>MAYRKRGARRETNLKQDERMQEKEDSKNINNDSPKSQLSEKVLSKKEEIITDNQEEVKISDEVKKSNKEESKQLLEVLKTKEEHQKEVQYEILQKTIPTFEPKESILKKLEDIKPEQAKKQTKLFRIFEPKQLPIYRANGERELRNRWYWKLKRDTLPDGDYDVREYFLNLYDQVLMEMPDYLLLKDMAVENKNSRDAGKVVDSETAAICDAIFQDEETEGAVRRFIAEMRQRVQADRNVVNYPSILHPIDHAFNEYFLQHQLVEPLNNDIIFNYIPERIRNDVNYILNMDRNLPSTARYIRPNLLQDRLNLHDNFESLWDTITTSNYILARSVVPDLKELVSTEAQIQKMSQDLQLEALTIQSETQFLTGINSQAANDCFKTLIAAMLSQRTMSLDFVTTNYMSLISGMWLLTVIPNDMFIRESLVACQLAIINTIVYPAFGMQRMHYRNGDPQTPFQIAEQQIQNFQVANWLHFVNYNQFRQVVIDGVLNQVLNDNIRNGHVVNQLMEALMQLSRQQFPTMPVDYKRSIQRGILLLSNRLGQLVDLTRLLSYNYETLMACITMNMQHVQTLTTEKLQLTSVTSLCMLIGNATVIPSPQTLFHYYNVNVNFHSNYNERINDAVAIITAANRLNLYQKKMKSIVEDFLKRLQIFDVARVPDDQMYRLRDRLRLLPVEIRRLDIFNLIAMNMEQIERASDKIAQGVIIAYRDMQLERDEMYGYVNIARNLDGFQQINLEELMRSGDYAQITNMLLNNQPVALVGALPFITDSSVISLIAKLDATVFAQIVKLRKVDTLKPILYKINSDSNDFYLVANYDWIPTSTTKVYKQVPQQFDFRASMHMLTSNLTFTVYSDLLAFVSADTVEPINAVAFDNMRIMNEL[2x];>MDVLYSLSKTLKDARDKIVEGTLYSNVSDLIQQFNQMIITMNGNEFQTGGIGNLPIRNWNFNFGLLGTTLLNLDANYVETARNTIDYFVDFVDNVCMDEMVRESQRNGIAPQSDSLRKLSAIKFKRINFDNSSEYIENWNLQNRRQRTGFTFHKPNIFPYSASFTLNRSQPAHDNLMGTMWLNAGSEIQVAGFDYSCAINAPANIQQFEHIVPLRRVLTTATITLLPDAERFSFPRVINSADGATTWFFNPVILRPNNVEVEFLLNGQIINTYQARFGTIVARNFDTIRLSFQLMRPPNMTPAVAVLFPNAQPFEHHATVGLTLRIESAVCESVLADASETLLANVTSVRQEYAIPVGPVFPPGMNWTDLITNYSPSREDNLQRVFTVASIRSMLIK[13x];>[13x]MYGIEYTTVLTFLISIILLNYILKSLTRIMDFIIYRFLFIIVILSPFLRAQNYGINLPITGSMDTAYANSTQEETFLTSTLCLYYPTEAATEINDNSWKDTLSQLFLTKGWPTGSVYFKEYTNIASFSVDPQLYCDYNVVLMKYDATLQLDMSELADLILNEWLCNPMDITLYYYQQTDEANKWISMGSSCTIKVCPLNTQTLGIGCLTTDATTFEEVATAEKLVITDVVDGVNHKLDVTTATCTIRNCKKLGPRENVAVIQVGGSDILDITADPTTAPQTERMMRINWKKWWQVFYTVVDYVDQIIQVMSKRSRSLNSAAFYYRV

The infectivity of rotavirus (RV), the leading cause of childhood diarrhea, hinges on the activation of viral particles through the proteolysis of the spike protein by trypsin-like proteases in the host intestinal lumen. The RV virion is an icosahedral triple layered particle in which the segmented viral genome and the polymerase complexes are packaged in a capsid made of the VP2 protein. The external layer is formed by trimers of the VP7 glycoprotein in phase with the underlaying VP6 shell and 60 trimeric VP4 spikes, which project from the VP7 layer, that clamps them and partially covers their base. This outer layer is responsible for the first steps of RV infection: attachment to cell surface receptors, lipid bilayer penetration, and release of the double-layered particle (DLP) into the cytosol, where transcription of the viral genome is initiated.

To obtain high-resolution maps of activated and inactivated particles, TLP from cells infected with rotavirus in the presence of trypsin (TR-TLP), or in its absence in medium supplemented with the protease inhibitor leupeptin (NTR-TLP), were purified by density gradient ultracentrifugation and characterized by SDS-PAGE. Three-dimensional reconstructions (3DR) of NTR- and TR-TLP were computed using SPA with imposition of icosahedral symmetry, achieving resolutions of 3.40 Å and 3.48 Å for NTR- and TR-TLP, respectively. The 3D architecture of the treated and untreated spikes showed a similar average density. However, the NTR spike was slightly shorter and wider than the TR spike, and had an additional density at the base, consistent with the lectin domain of the VP4-C subunit previously described in these particles. While the density of the VP2, VP6 and VP7 shells exhibited a homogeneous high local resolution, the spike showed a radial decrease in resolution as it extended away from the outer shell surface, with particularly low resolution in the body and head regions. In addition, although the VP4-C lectin domain was detected, it was observed with low density, which has been associated with flexibility. These limitations hinder the construction of reliable VP4 atomic coordinates in the spike density and require further density improvement for accurate interpretation. The resulting maps provided sufficient quality to support full atomic modelling in the foot and stalk domains, while in the body and head regions, a combination of backbone tracing and rigid-body fitting was applied (representative examples of model-to-map fitting for each region are shown in S8 Fig). These enhanced densities, together with the icosahedral 3DR of the complete NTR and TR TLPs, were used to build and refine the full asymmetric subunits, including all VP2, VP4, VP6, and VP7 chains.N,N-dimethylpyridine-3-sulfonamide | C7 H10 N2 O2 S | 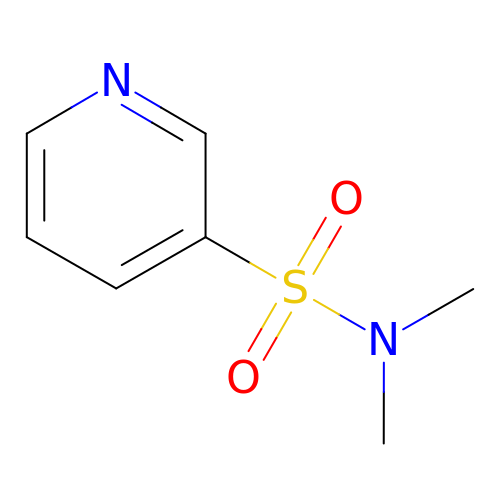HGZULNNLLFYOFI-UHFFFAOYSA-N Multidrug resistance protein 1 (MRP1) is an ATP-binding cassette (ABC) transporter that harnesses the energy of ATP to extrude substrates from the cytosol to the extracellular space. Native substrates of MRP1 include a variety of antioxidants, pro-inflammatory molecules, and hormones. MRP1 also transports a number of chemotherapeutic agents, thereby conferring drug resistance in acute myeloblastic and lymphoblastic leukemia, non-small-cell lung cancer, prostate cancer, breast cancer, and neuroblastoma. MRP1 is a single polypeptide comprising three transmembrane domains (TMD0, TMD1, and TMD2) and two cytosolic nucleotide-binding domains (NBD1 and NBD2).

Guided by the smFRET results, we then used cryo-EM to capture the most abundant structural configuration of wild-type (WT) MRP1 during active turnover. To prepare the sample for cryo-EM, WT bMRP1 (30 µM) was incubated with 80 µM LTC4 and 10 mM ATP-Mg2+ on ice for 10 min before plunge freezing in liquid ethane. On ice, we expect a slower turnover rate and thus even less depletion of ATP. This approximates an ‘active turnover’ condition where ATP hydrolysis has reached steady state. We first used all 1,143,729 particles from the cryo-EM dataset to calculate a 3.4 Å reconstruction that represents the dominant structure under the active turnover condition. Consistent with the single-molecule data, the resulting map shows an NBD-dimerized conformation, with an ATP molecule in the degenerate site and an ADP molecule in the consensus site. To improve the resolution of the structure, we also carried out 3D classification and obtained a higher quality map at 3.2 Å from a subset of the particles (Figure 6—figure supplements 1 and 2), which unambiguously shows an ADP molecule at the consensus site. Other than ADP occupying the consensus site in place of ATP, the overall structure of this post-hydrolysis conformation is essentially identical to that of the pre-hydrolytic structure solved with the hydrolysis-deficient E1454Q mutant (Johnson and Chen, 2018). In both structures, the intracellular gate is closed and the substrate-binding site is pulled apart such that LTC4 is no longer bound. Thus, for MRP1, ATP hydrolysis per se and the subsequent release of inorganic phosphate (Pi) do not induce conformational rearrangements.

> MALRDFCSVDGSDLFWEWNVTWNTSNPDFTKCFQNTVLVWVPCSYLWVCFPFYFLYLSHHDRGYIQMTHLNKAKTALGFLLWIVCWADLFYSFWERSMGKLLAPVFLVSPTLLGITMLLATFLIQIERRRGVQSSGIMLTFWLIALLCALAILRSKIMTALKEDARVDVFRDVTFYIYFSLVLIQLVLSCFSDRSPLFSETINDPNPCPESSASFLSRITFWWITGMMVQGYRQPLESTDLWSLNKEDTSEQVVPVLVKNWKKECAKSRKQPVKIVYSSKDPAKPKGSSKVDVNEEAEALIVKCPQKERDPSLFKVLYKTFGPYFLMSFLFKAVHDLMMFAGPEILKLLINFVNDKKAPEWQGYFYTALLFISACLQTLVLHQYFHICFVSGMRIKTAVIGAVYRKALVITNAARKSSTVGEIVNLMSVDAQRFMDLATYINMIWSAPLQVILALYLLWLNLGPSVLAGVAVMVLMVPLNAVMAMKTKTYQVAHMKSKDNRIKLMNEILNGIKVLKLYAWELAFKDKVLAIRQEELKVLKKSAYLAAVGTFTWVCTPFLVALSTFAVYVTVDENNILDAQKAFVSLALFNILRFPLNILPMVISSIVQASVSLKRLRVFLSHEDLDPDSIQRRPIKDAGATNSITVKNATFTWARNDPPTLHGITFSVPEGSLVAVVGQVGCGKSSLLSALLAEMDKVEGHVTVKGSVAYVPQQAWIQNISLRENILFGRQLQERYYKAVVEACALLPDLEILPSGDRTEIGEKGVNLSGGQKQRVSLARAVYCDSDVYLLDDPLSAVDAHVGKHIFENVIGPKGLLKNKTRLLVTHAISYLPQMDVIIVMSGGKISEMGSYQELLARDGAFAEFLRTYASAEQEQGQPEDGLAGVGGPGKEVKQMENGMLVTDTAGKQMQRQLSSSSSYSRDVSQHHTSTAELRKPGPTEETWKLVEADKAQTGQVKLSVYWDYMKAIGLFISFLSIFLFLCNHVASLVSNYWLSLWTDDPIVNGTQEHTQVRLSVYGALGISQGITVFGYSMAVSIGGIFASRRLHLDLLHNVLRSPISFFERTPSGNLVNRFSKELDTVDSMIPQVIKMFMGSLFNVIGACIIILLATPMAAVIIPPLGLIYFFVQRFYVASSRQLKRLESVSRSPVYSHFNETLLGVSVIRAFEEQERFIRQSDLKVDENQKAYYPSIVANRWLAVRLECVGNCIVLFASLFAVISRHSLSAGLVGLSVSYSLQVTTYLNWLVRMSSEMETNIVAVERLKEYSETEKEAPWQIQDMAPPKDWPQVGRVEFRDYGLRYREDLDLVLKHINVTIDGGEKVGIVGRTGAGKSSLTLGLFRIKESAEGEIIIDDINIAKIGLHDLRFKITIIPQDPVLFSGSLRMNLDPFSQYSDEEVWTSLELAHLKGFVSALPDKLNHECAEGGENLSVGQRQLVCLARALLRKTKILVLDEATAAVDLETDDLIQSTIRTQFDDCTVLTIAHRLNTIMDYTRVIVLDKGEIQEWGSPSDLLQQRGLFYSMAKDSGLVSNSLEVLFQ> HHHHHHMIIKNYSYARQNLKALMTKVNDDSDMVTVTSTDDKNVVIMSESDYNSMMETLYLQQNPNNAEHLAQSIADLERGKTI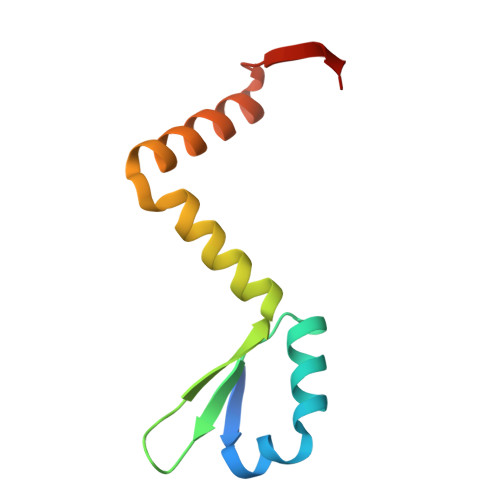TKDIDV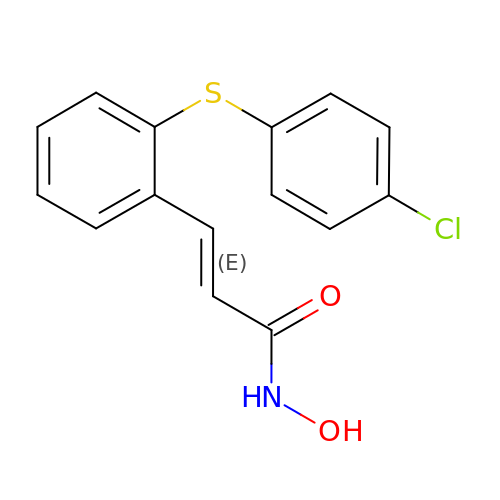(~{E})-3-[2-(4-chlorophenyl)sulfanylphenyl]-~{N}-oxidanyl-prop-2-enamide | C15 H12 Cl N O2 S | LOPNSVKBMZZEHH-BJMVGYQFSA-N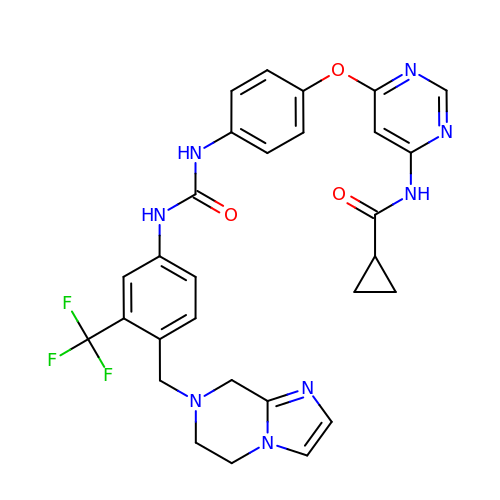N-(6-(4-(3-(4-((5,6-dihydroimidazo[1,2-a]pyrazin-7(8H)-yl)methyl)-3-(trifluoromethyl)phenyl)ureido)phenoxy)pyrimidin-4-yl)cyclopropanecarboxamide | C29 H27 F3 N8 O3 | JVAUXOQNQAAUBJ-UHFFFAOYSA-N>[6x]APKRKAGVSKCETKC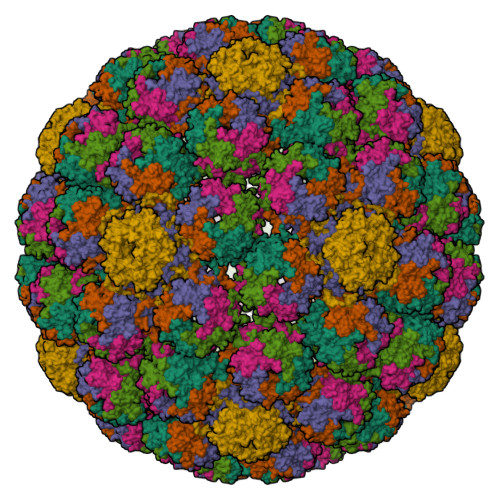TKACPRPAPVPKLLIKGGMEVLDLVTGPDSVTEIEAFLNPRMGQPPTPESLTEGGQYYGWSRGINLATSDTEDSPGNNTLPTWSMAKLQLPMLNEDLTCDTLQMWEAVSVKTEVVGSGSLLDVHGFNKPTDTVNTKGISTPVEGSQYHVFAVGGEPLDLQGLVTDARTKYKEEGVVTIKTITKKDMVNKDQVLNPISKAKLDKDGMYPVEIWHPDPAKNENTRYFGNYTGGTTTPPVLQFTNTLTTVLLDENGVGPLCKGEGLYLSCVDIMGWRVTRNYDVHHWRGLPRYFKITLRKRWVKNPYPMASLISSLFNNMLPQVQGQPMEGENTQVEEVRVYDGTEPVPGDPDMTRYVDRFGKTKTVFPGN> LAPNDPYYQAYQWHLHNATGGINAPSAWDVSQGEGVVVAVLDTGILPQHPDLVGNLLEGYDFISDAATSRRATNDRVPGAQDYGDWVENDNECYTGSVAEDSSWHGTHVAGTVAEQTNNGVGMAGVAHKAKVLPVRVLGKCGGYLSDIADAITWASGGTVAGVPANANPAEVINMSLGGSGSCDGTYQDAINGAISRGTTVVVAAGNETDNASKYRPASCDGVVTVGATRITGGITYYSNYGSRVDLSGPGGGGSVDGNPGGYVWQSGSDAATTPESGSYSYMGMGGTSMASPHVAAVAALVQSALIAAGKDPLAPAAMRTLLKETARPFPVSIPTATPIGTGIVDAKAALAAALE

Through the COVID-19 pandemic it gained more prominence by being a key pathogen in respiratory co-infections. This study will present a structural analysis of StmPr1, S. maltophilia’s main virulence factor, an excreted serine protease. StmPr1 is a member of the subtilases family defined by Siezen & Leunissen et al.. It shows the main structural and functional elements of the family, such as a reactive triad consisting of Asp42, His105, and Ser28922. The catalytic triad consisting of Asp42, His105, and Ser289 is located on top of β1 (Asp42), α4 (His105), and α10 (Ser289).

StmPr1’s 36 kDa structure, solved and analyzed by x-ray crystallography, shares structural similarities with other subtilases, first described by Wright et al. for subtilisin BPN’24. StmPr1 has the subtilase-typical α/β fold formed by seven, instead of eight, parallel β-sheets with five α-helices surrounding the sheets where four helices are antiparallel to the sheets. Besides the seven parallel β-sheets forming the core, StmPr1 shows only antiparallel β-sheet formations in β2/β3, β6/β8, and β11/β12, all located on the fringes of the structure and therefore supporting the structural stability in most loop-rich regions of the protein. The protein also has two disulfide bonds, Cys93 - Cys141 and Cys183 - Cys220. Cys93-Cys141 links the loop connecting β1 and α5 to a loop covering the catalytic triad, beginning directly behind β3 at Gly79 and going to Ser103 on top of α4. Thereby, it strengthens the connection of the loop to the core structure helping to form a kind of lid above the substrate binding cleft. This lid is a loop insertion, not present in subtilisin BPN’24 Proteinase K26 Thermitase27 or subtilisin Carlsberg28. The lid may facilitate and support two distinct functions, on the one hand, the lid may move to block the entry into the substrate binding cleft, thereby preventing unwanted binding to the catalytic triad. On the other hand, closing it also stabilizes potential substrates inside the substrate-binding cleft. The StmPr1 protease exhibits some special and additional structural features, like a relatively high content of Glu and Asp residues and a relatively low content of Arg and Lys residues on the surface, which may give the enzyme the ability to be active in an alkaline environment.> STRE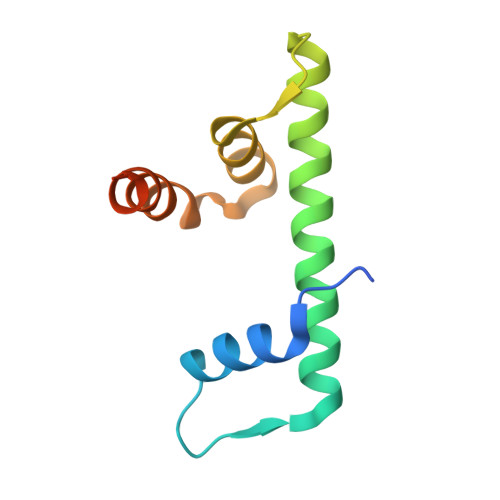QDRFLPIANVSRIMKKALPANAKISKDAKETVQECVSEFISFITGEASDKCQREKRKTINGDDLLWAMTTLGFEDYVEPLKVYLQKYREVEGEKTTTAG>[2x]GSHMALALVGEKIDRNRFTGEKIENSTFFNCDFS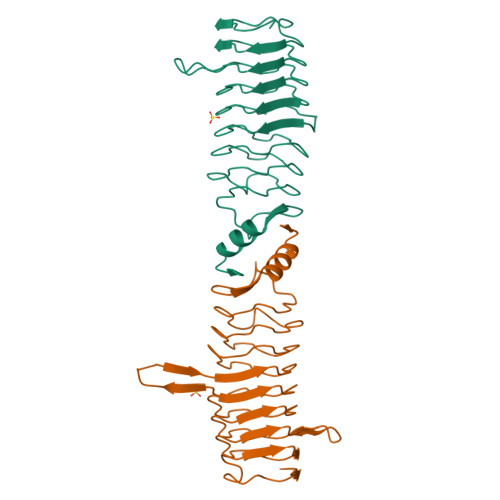GADLSGTEFIGCQFYDRESQKGCNFSRAMLKDAIFKSCDLSMADFRNSSALGIEIRHCRAQGADFRGASFRNMITTRTWFCSAYITNTNLSYANFSKVVLEKCELWENRWIGAQVLGATFSGSDLSGGEFSTFDWRAANFTHCDLTNSELGDLDIRGVDLQGVKLDNYQASLLMERLGIAVIG>MINYSERIPNNVNLNENKTLQRALEQWQPSFLNWWDDMGPENSSNYDVYLRTAVSVDPKGWADFGYVKMHDYRWGIFLAPQEGEKKITFGEHKGQDVWQEVPGEYRSTLRRIIVTQGDTEPASVEQQRHLGLTAPSLYDLRNLFQVNVEEGRHLWAMVYLLHAHFGRDGREEGEALLERRSGDEDNPRILTAFNEKTPDWLSFFMFTFITDRDGKFQLASLAESAFDPLARTCKFMLTEEAHHLFVGESGIARVIQRTCEVMKELGTDDPAKLRAAGVIDLPTLQKYLNFHYSVTSDLYGAEISSNAATYYTNGLKGRFEEEKIGDDHKLQNSEYEVMDVAGDKILTRHVPALSALNERLRDDWITDVQAGVDRWNRIPAKFG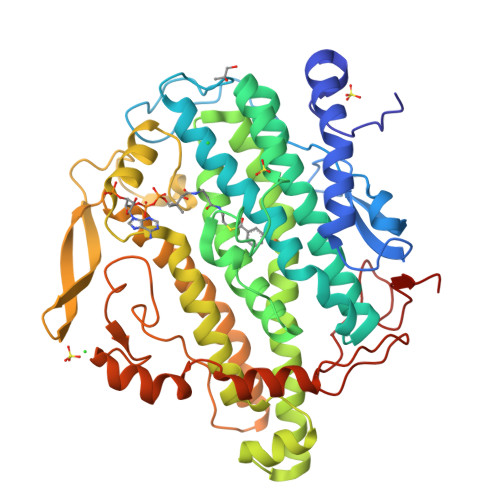FDFRFTLPHKGFHRKIGMFADVHVSPDGRLISEAEWTHQHKNWLPTESDRLYVHSLMGRCLEPGKFANWIAAPARGINNQPVNFEYVRFNWSHPQFEK[4x]N-carbamimidoyl-L-glutamic acid | C6 H11 N3 O4 | 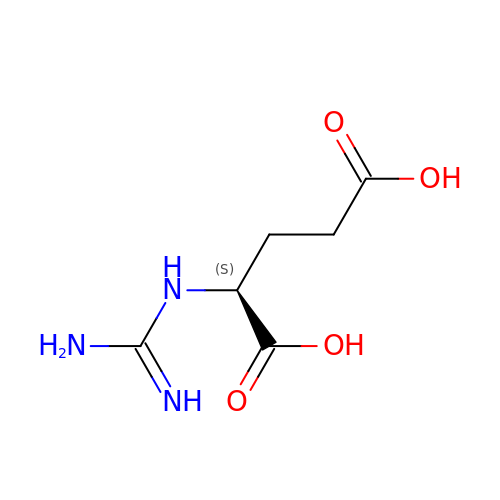RHVVRMJOHATSPD-VKHMYHEASA-N> MLAQVLRRQALQHVRLARAAAPSLTRWYASYPPHT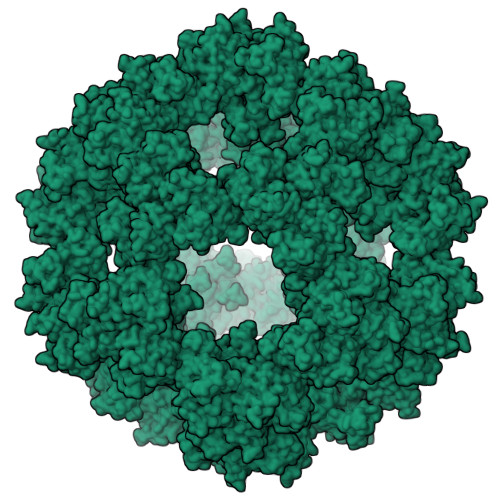IVKMPALSPTMTSGNIGAWQKKPGDAITPGEVLVEIETDKAQMDFEFQEEGVLAKILKETGEKDVAVGSPIAVLVEEGTDINAFQNFTLEDAGGDAAAPAAPAKEELAKAETAPTPASTSAPEPEETTSTGKLEPALDREPNVSFAAKKLAHELDVPLKALKGTGPGGKITEEDVKKAASAPAAAAAAPGAAYQDIPISNMRKTIATRLKESVSENPHFFVTSELSVSKLLKLRQALNSSAEGRYKLSVNDFLIKAIAVACKRVPAVNSSWRDGVIRQFDTVDVSVAVATPTGLITPIVKGVEAKGLETISATVKELAKKARDGKLKPEDYQGGTISISNMGMNPAVERFTAIINPPQAAILAVGTTKKVAVPVENEDGTTGVEWDDQIVVTASFDHKVVDGAVGAEWMRELKKVVENPLELLL> XYIQ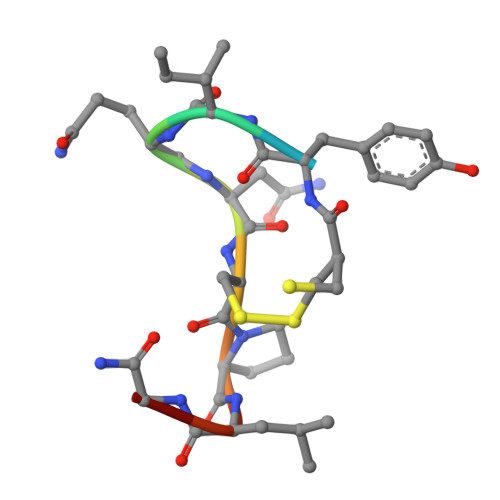NCPLGX>TMAHHHHHHVTNSTDGRADGRLRVVVLGSTGSIGTQALQVIADNPDRFEVVGLAAGGAHLDTLLRQRAQTGVTNIAVADEHAAQRVGDIPYHGSDAATRLVEQTEADVVLNALVGALGLRPTLAALKTGARLALANKESLVAGGSLVLRAARPGQIVPVDSEHSALAQCLRGGTPDEVAKLVLTASGGPFRGWSAADLEHVTPEQAGAHPTWSMGPMNTLNSASLVNKGLEVIETHLLFGIPYDRIDVVVHPQSIIHSMVTFIDGSTIAQASPPDMKLPISLALGWPRRVSGAAAACDFHTASSWEFEPLDTDVFPAVELARQAGVAGGCMTAVYNAANEEAAAAFLAGRIGFPAIVGIIADVLHAADQWA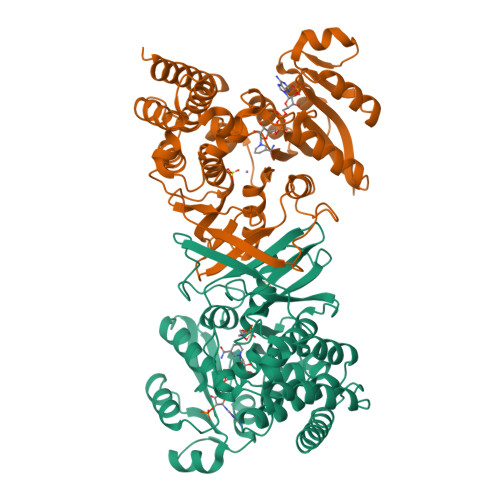VEPATVDDVLDAQRWARERAQRAVSGM[2x]> ASWQDYHSEFSKKYGD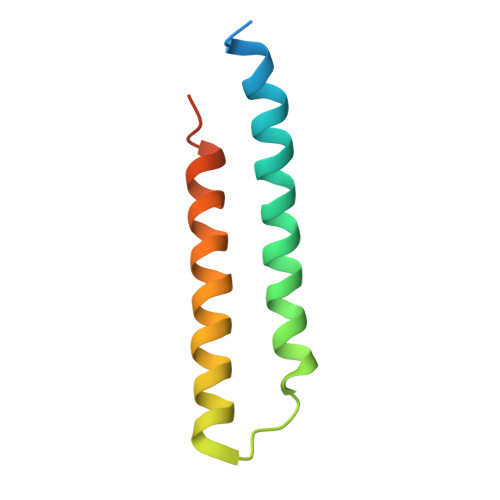IALKKKLEQNTKKLDEESSQLETTTRSIDSADDLDQFIKNYLDIRTQYHLRREKLATWDKQGNLKY> GSMEAVLNEL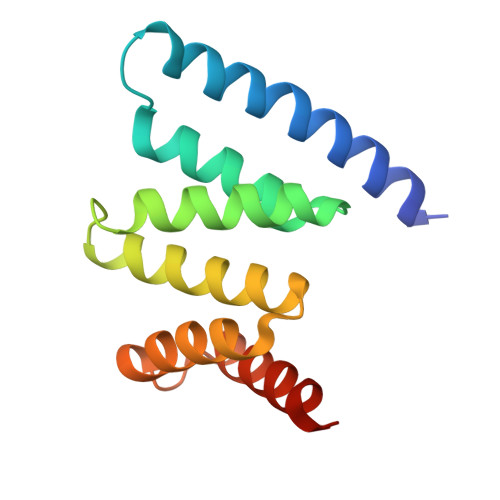VSVEDLLKFEKKFQSEKAAGSVSKSTQFEYAWCLVRSKYNDDIRKGIVLLEELLPKGSKEEQRDYVFYLAVGNYRLKEYEKALKYVRGLLQTEPQNNQAKELERLIDKAMKKDGL> PTGNNAEICLLPLDYGPCRALLLRYYYDRYTQSCRQFLYGGCEGNANNFYTWEACDDA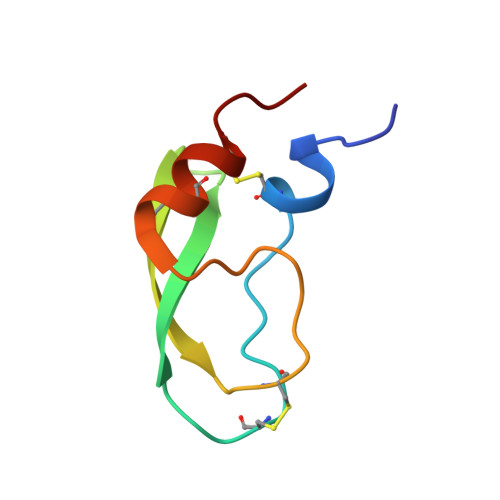CWRIE> GGCGCUG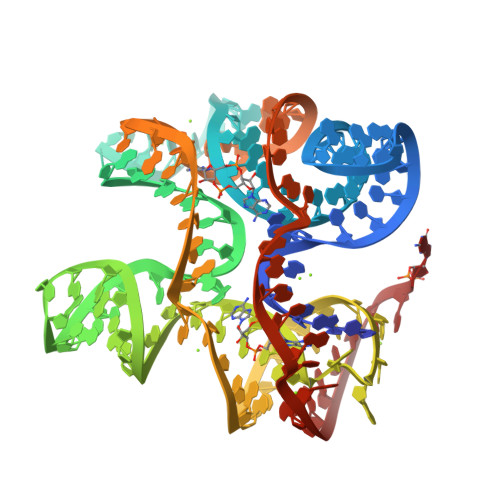AAUUCCCUGAAGGGAAACGGGGGACCCAAUCUUCAGGGGUGAAUCCCACGUAAGUGGGUAGGGCUAGUCUCUUUCGGCCCGAACCCGUCAGCUAACCUCGUAAGCGUGGAAAGAGGX> GSHMNVAEISS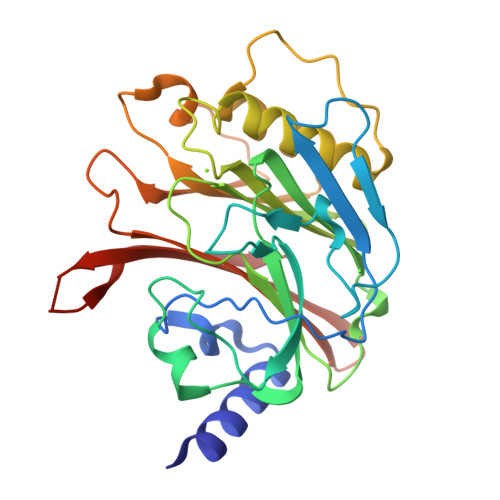INFRRLNSGNINVLKGRGVFSSRRLREIYLRFDAANADELRPGDVYVKKTKFDSMGYDSHFYNEGIGINGAPTLNTYTGEYVADSSSQGATYWLKYNLTNETSIIKVSNSARGANGIKIALEEIEENKPVVITSGTLTGCTVVFARKGEYFYAVHTGNSESLIGFTSTSGVAKAIEVLSSLSELEVPALPDVINNNTLVEYLSDNFDSALISYSSSSLKPNSMINISRENVSTFSYYTDDIQLPSFGTSVTILVRTNDNTVVRSLSESYTMNSNSSKMVVFNVLQKDF>[4x]SIGVSDGLLSYIKNENENKGFLGIYGFFTGADKNIEKATLYKNLIAKYQNNHFISLIILSALVSDSKTPLMTQYLVGYLDFPSKALLANKITELLLKELENPDMREILGSRLATDVIEELETKIIRYIHNPAGSDIHSTLNLWTADKIKAATNSSLTI

While SidM catalyzes the attachment of adenosine monophosphate (AMP) to Rab1, SidD catalyzes AMP removal from Rab1, a process known as deAMPylation. Inactivation and removal of Rab1 is initiated upon translocation of the effector SidD which deAMPylates Rab1, thereby priming it for inactivation by the L. pneumophila GAP LepB and causing its gradual removal from the LCV 4–6 hours after bacterial uptake. SidD is a protein of 507 amino acids with no significant sequence homology to other entries in the database. Taken together, our data revealed that the CTD mediates localization of SidD to membranes using a dual-binding mode that combines a general membrane-binding determinant in form of the loopCTD with a specificity determinant represented by a helix-turn-helix unit at the C-terminus.

Thus, we focused on obtaining a higher-resolution crystal structure of the CTD alone. The construct encompassing amino acids 350–507 (SidD350-507) crystallized readily and diffracted well. The structure was solved by single-wavelength anomalous diffraction using selenium as the anomalous scatterer. The model was refined to a resolution of 2.5 Å (Rwork 26.4%, Rfree 28.7%) with good stereochemistry. Residues 350–367 and residues 496–507 have been excluded from the final model as they were located in areas of poor-quality electron density and were most likely disordered. The structure of SidD350-507 revealed a compact helical domain where a central helix (α9) forms the hydrophobic core that is surrounded by five helices that are tilted with respect to the central one and form an antiparallel bundle. Despite extensive in silico analyses, we were able to only find domains or regions with weak structural homology to SidD350-507. Automated ion placement in PHENIX.REFINE identified a hexa-coordinated Mg2+ with the classical octahedral geometry formed by the Oδ atoms of T417, T421, the main chain carbonyl oxygens of L411, V412, and D414, and one water molecule. In addition, upon closer inspection of this region we found a second metal ion, which despite not having a recognizable coordination shell, was identified as Zn2+ based on the clear Zn peaks in anomalous difference Fourier maps from data collected at the zinc edge. Given their selective retention during protein production in and purification from E. coli, we cannot exclude the possibility that they contribute to structural stability of SidD or possibly even a yet undefined catalytic activity.> MVGQIAKEMGLRAYIVGGVVRDILLGKEVWDVDFVVEGNAIELAKELARRHGVNVHPF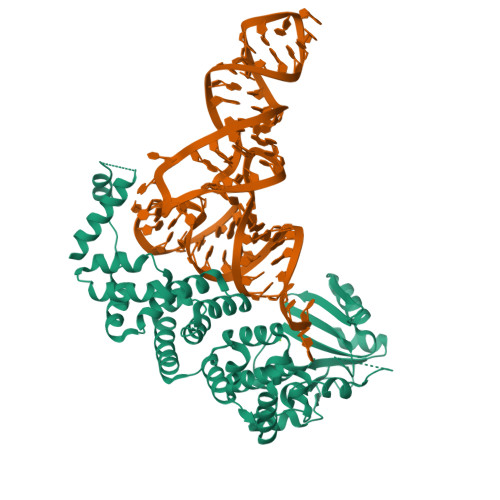PEFGTAHLKIGKLKLEFATARRETYPRPGAYPKVEPASLKEDLIRRDFTINAMAISVNLEDYGTLIDYFGGLRDLKDKVIRVLHPVSFIEDPVRILRALRFAGRLNFKLSRSTEKLLKQAVNLGLLKEAPRGRLINEIKLALREDRFLEILELYRKYRVLEEIIEGFQWNEKVLQKLYALRKVVDWHALEFSEERIDYGWLYLLILISNLDYERGKHFLEEMSAPSWVRETYKFMKFKLGSLKEELKKAKENYEVYRLLKPLHTSVLLLLMLEEELKEKIKLYLEKLRKVKLPKEKIEELKKQGLKGKELGERIEELKREIMNKIKLAAALEHHHHHH>[2x]EWQENKSWNAHFTEHKSQGVVVLWNENKQQGFTNNLKRANQAFLPASTFKIPNSLIALDLGVVKDEHQVFKWDGQTRDIATWNRDHNLITAMKYSVVPVYQEFARQIGEARMSKMLHAFD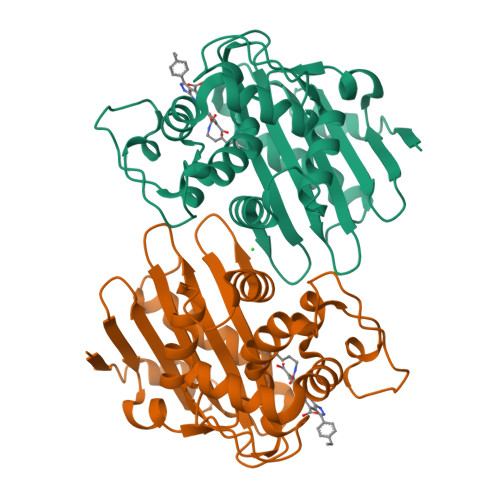YGNEDISGNVDSFWLDGGIRISATEQISFLRKLYHNKLHVSERSQRIVKQAMLTEANGDYIIRAKTGYSTRIEPKIGWWVGWVELDDNVWFFAMNMDMPTSDGLGLRQAITKEVLKQEKIIP>MSQRITIDPVTRIEGHLRIDCEIENGVVSKAWASGTMWRGMEEIVKNRDPRDAWMIVQRICGVCTTTHALSSVRAAESALNIDVPVNAQYIRNIILAAHTTHDHIVHFYQLSALDWVDITSALQADPTKASEMLKGVSTWHLNSPEEFTKVQNKIKDLVASGQLGIFANGYWGHPAMKLPPEVNLIAVAHYLQALESQRDANRVVALLGGKTPHIQNLAVGGVANPINLDGLGVLNLERLMYIKSFIDKLSDFVEQVYKVDTAVIAAFYPEWLTRGKGAVNYLSVPEFPTDSKNGSFLFPGGYIENADLSSYRPITSHSDEYLIKGIQESAKHSWYKDEAPQAPWEGTTIPAYDGWSDDGKYSWVKSPTFYGKTVEVGPLANMLVKLAAGRESTQNKLNEIVAIYQKLTGNTLEVAQLHSTLGRIIGRTVHSSELQDILQNQYSALITNIGKGDHTTFVKPNIPATGEFKGVGFLEAPRGMLSHWMVIKDGIISNYQAVVPSTWNSGPRNFNDDVGPYEQSLVGTPVADPNKPLEVVRTIHSFDPCMACAVHVVDADGNEVVSVKVL[2x];>EMAESVTNPQRPPVIWIGAQECTGCTESLLRATHPTVENLVLETISLEYHEVLSAAFGHQVEENKHNALEKYKGQYVLVVDGSIPLKDNGIYCMVAGEPIVDHIRKAAEGAAAIIAIGSCSAWGGVAAAGVNPTGAVSLQEVLPGKTVINIPGCPPNPHNFLATVAHIITYGKPPKLDDKNRPTFAYGRLIHEHCERRPHFDAGRFAKEFGDEGHREGWCLCHLGCKGPETYGNCSTLQFCDVGGVWPVAIGHPCYGCNEEGIGFHKGIHQLANVENQTPRSQKP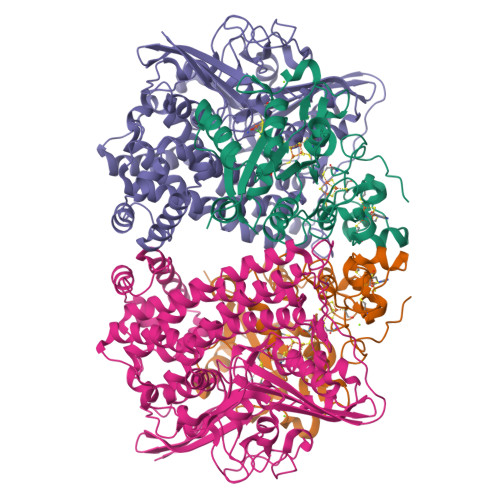DVNAKEGGNVSRSHHHHHH[2x]> MAAFKPNSINYILGLDIGIASVGWAMVEIDEEENPIRLIDLGVRVFERAEVPKTGDSLAMARRLARSVRRLTRRRAHRLLRTRRLLKREGVLQAANFDENGLIKSLPNTPWQLRAAALDRKLTPLEWSAVLLHLIKHRGYLSQRKNEGETADKELGALLKGVAGNAHALQTGDFRTPAELALNKFEKESGHIRNQRSDYSHTFSRKDLQAELILLFEKQKEFGNPHVSGGLKEGIETLLMTQRPALSGDAVQKMLGHCTFEPAEPKAAKNTYTAERFIWLTKLNNLRILEQGSERPLTDTERATLMDEPYRKSKLTYAQARKLLGLEDTAFFKGLRYGKDNAEASTLMEMKAYHAISRALEKEGLKDKKSPLNLSPELQDEIGTAFSLFKTDEDITGRLKDRIQPEILEALLKHISFDKFVQISLKALRRIVPLMEQGKRYDEACAEIYGDHYGKKNTEEKIYLPPIPADEIRNPVVLRALSQARKVINGVVRRYGSPARIHIETAREVGKSFKDRKEIEKRQEENRKDREKAAAKFREYFPNFVGEPKSKDILKLRLYEQQHGKCLYSGKEINLGRLNEKGYVEIDHALPFSRTWDDSFNNKVLVLGSENQNKGNQTPYEYFNGKDNSREWQEFKARVETSRFPRSKKQRILLQKFDEDGFKERNLNDTRYVNRFLCQFVADRMRLTGKGKKRVFASNGQITNLLRGFWGLRKVRAENDRHHALDAVVVACSTVAMQQKITRFVRYKEMNAFDGKTIDKETGEVLHQKTHFPQPWEFFAQEVMIRVFGKPDGKPEFEEADTLEKLRTLLAEKLSSRPEAVHEYVTPLFVSRAPNRKMSGQGHMETVKSAKRLDEGVSVLRVPLTQLKLKDLEKMVNREREPKLYEALKARLEAHKDDPAKAFAEPFYKYDKAGNRTQQVKAVRVEQVQKTGVWVRNHNGIADNATMVRVDVFEKGDKYYLVPIYSWQVAKGILPDRAVVQGKDEEDWQLIDD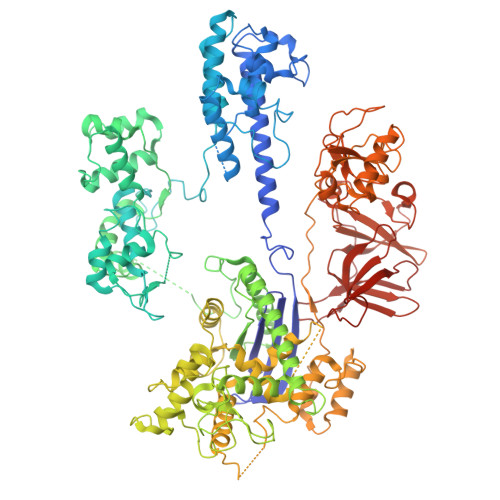SFNFKFSLHPNDLVEVITKKARMFGYFASCHRGTGNINIRIHDLDHKIGKNGILEGIGVKTALSFQKYQIDELGKEIRPCRLKKRPPVR>GSIIEMRDVVKKYDNGTTALRGVSVSVQPGEFAYIVGPSGAGKSTFIRSLYREVKIDKGSLSVAGFNLVKIKKKDVPLLRRSVGVVFQDYKLLPKKTVYENIAYAMEVIGENRRNIKRRVMEVLDLVGLKHKVRSFPNELSGGE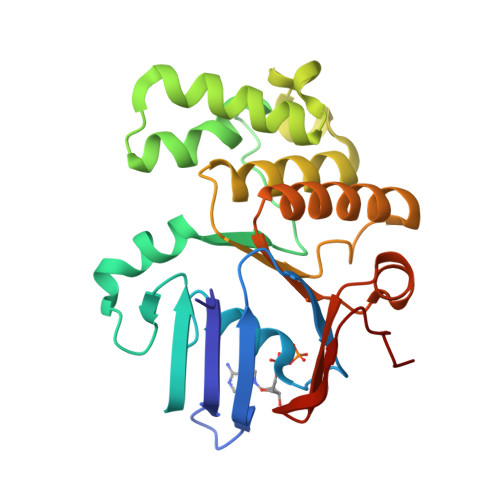QQRIAIARAIVNNPKVLIADEPTGNLDPDNSWEIMNLLERINLQGTTILMATHNSQIVNTLRHRVIAIENGRVVRDESKGEYGYDD[3x]> MLLCLLYFTSSWCSEADVPDVCTNSGMIAINFVDGPVRGVTDRILNTLDELGVKATFSFTVNQKAVGNVGQLYRRAVEEGHNVALRVDPSMDEGYQCLSQDALENNVDREIDTIDGLSGTEIRYAAVPICNGQVNSEMYNILTERGVLPVGYTFCPYDYDDPVGEFESMIEGSDPKH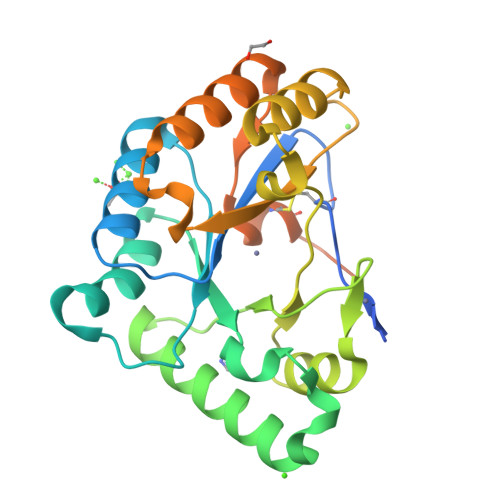HSFIILMHDGQEADTSRLENMVKIGKDKGYRFVNMDECLQGYKGAPGDPELSLRGKGVESIGKGFLPFFLMMLVRLL> SEGNGPAAVHYQPASPPRDACVYSSCYCEENVWKLCEYIKNHDQYPLEECYAVFISNERKMIPIWKQQARPGDGPVIWDYHVVLLHVSSGGQSFIYDLDTVLPFPCLFDTYVEDAIKSDDDIHPQFRRKFRVICADSYLKNFASDRSHMKDSSGNWREPPPPYPCIETGDSKMNLNDFISMDPKVGWGAVYTLSEFTHRFGS

The human C8orf32 gene encodes human N-terminal glutamine amidohydrolase isoform 1 (hNtaq1). Ntaq is an initial component of the N-end rule pathway and converts N-terminal glutamine to glutamate. In the N-end rule pathway, N-terminal glutamine and asparagine are tertiary destabilizing residues and these residues are converted into secondary destabilizing N-terminal glutamate and aspartate by deamidation. The N-terminal amidohydrolases are classified into the N-terminal glutamine amidohydrolase (Ntaq) and the N-terminal asparagine amidohydrolase (Ntan), which share low amino acid sequence identity and mediate the deamidation of N-terminal glutamine and asparagine, respectively.

In order to understand the relationship between the structure and function of hNtaq1, we determined the crystal structure of recombinant hNtaq1 bound with the adjacent N-terminus of a symmetry-related hNtaq1 molecule at 1.5 Å resolution. The hNtaq1 protein contains 205 amino acids, of which 202 have been successfully modeled in the presented hNtaq1 structure. Three C-terminal residues (Lys203, Asn204, and Cys205) were disordered in the crystal and could not be modeled. free values of the final refined model were 14.4% and 17.0%, respectively. hNtaq1 is a monomeric globular protein with a novel structural fold of alpha-beta-alpha three-layer sandwich architecture. The catalytic triad (Cys28, His81, and Asp97) is highly conserved among Ntaq proteins, transglutaminases, and cysteine proteases of diverse organisms. In the structure of hNtaq1, Asp97 forms hydrogen bonds with His81, Tyr111 and a water molecule 1 (water403 in PDB) and His81 interacts with another water molecule 2 (water444 in PDB) via hydrogen bond. The N-terminus of a symmetry-related monomer is anchored into the active site of hNtaq1 with the side chain of the N-terminal residue (Ser1) in close proximity of the catalytic Cys28. The surface charge of the binding cleft is predominantly negative, and several hydrophobic and aromatic residues (Val76, Ile77, Tryp78, and Tyr80) are well oriented to recognize main chain backbone of the substrate-mimicking peptide and to stabilize aliphatic part of the bound substrate-mimicking peptide. Overall, the active site bound with the substrate-mimicking peptide directly suggests possible interaction mode of hNtaq1 with substrates.>[2x]MAVNSKYHHSCINCGGLNTDERNERGLPCEVCLPEDSPSDIYRALLERKTLKEYRFYHEFWNEYEDFRSFFKKKFGKDLTGYQRLWAKRIVQGKSFTMVAPTGVGKTTFGMMTALWLARKGKKSALVFPTVTLVKQTLERLQKLADEKVKIFGFYSSMKKEEKEKFEKSFEEDDYHILVFSTQFVSKNREKLSQKRFDFVFVDDVDAVLKASRNIDTLLMMVGIPEEIIRKAFSTIKQGKIYERPKNLKPGILVVSSATAKPRGIRPLLFRDLLNFTVGRLVS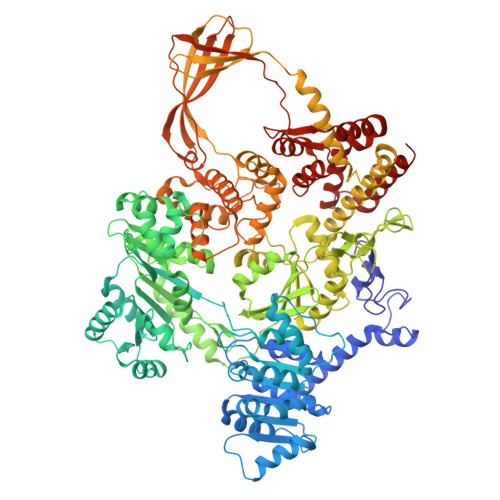VARNITHVRISSRSKEKLVELLEIFRDGILIFAQTEEEGKELYEYLKRFKFNVGETWSEFEKNFEDFKVGKINILIGVQAYYGKLTRGVDLPERIKYVIFWGTPSMRFSLELDKAPRFVLARVLKEMGLIKAQENPDVEELRKIAKEHLTQKEFVEKVKEMFRGVVVKDEDLELIIPDVYTYIQASGRSSRILNGVLVKGVSVIFEEDEEIFESLKTRLLLIAEEEIIEEAEANWKELVHEVEESRRRSERELTDTSRSLLIIVESPTKAETLSRFLGRASSRKERNIIVHEAVTGEGVILFTATRGHVYDLVTKGGIHGVEEENGKFVPVYNSLKRCRDCGYQFTEDRDECPVCSSKNIDDKTETLRALREISLEADEILVATDPDVEGEKISWDVTQYLLPSTRSLRRIEMHEITRYGFKKARESVRFVDFNLVKAQIVRRVQDRWIGFELSGKLQKRFGRSNLSAGRVQSTVLGWIVEREEEYKKSEKDFTLLVLENGVNLEVEGKIADDVVTVVELQEAEEEKNPLPPYTTSSALSEISQKLRLGVQEVMDILQDLFEKGFITYHRTDSTRISLEGQNVARTYLRKIGKEDIFMGRSWSTEGAHEAIRPVKPIDARELEEMIEEGLIADLTKKHLRVYELIFNRFLASQSAAVKVKKQIVTVDVDGKRMGIEQIVEILRDGWNLFVPLTVSPRFEHRTYKIKEKKFYKKHTVPLFTQASIVEEMKKRGIGRPSTYAKIVEVLFRRGYVYEDKYKRVRPTRFGVMVYSYLKERYEKYVTEETTRRLEEIMDKVERGEEDYQATLRLLYEEIKSLMEEG>[2x]MVLYFIGLGLYDERDITVKGLEIAKKCDYVFAEFYTSLMAGTTLGRIQKLIGKEIRVLSREDVEL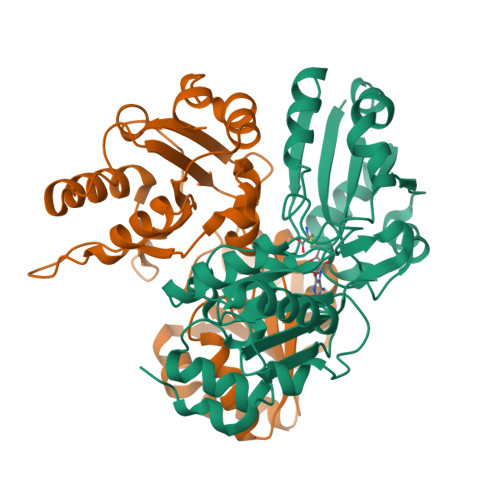NFENIVLPLAKENDVAFLTPGDPLVATTHAELRIRAKRAGVESYVIHAPSIYSAVGITGLHIYKFGKSATVAYPEGNWFPTSYYDVIKENAERGLHTLLFLDIKAEKRMYMTANEAMELLLKVEDMKKGGVFTDDTLVVVLARAGSLNPTIRAGMVKDLIREDFGDPPHILIVPGKLHIVEAEYLVEIAGAPREILRVNV ETHENO-NAD | C23 H27 N7 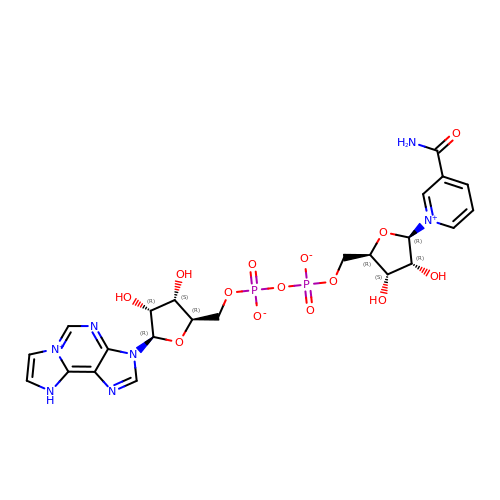O14 P2 | JCDBQDNBEQHDHK-BSLNIGMPSA-N> FVRKNPKSDKFKVKRFHHIEFWCGDATNVARRFSWGLGMRFSAKSDLSTGNMVHASYLLTSGDLRFLFTAPYSPSLSAGEIKPTTTASIPSFDHGSCRSFFSSHGLGVRAVAIEVEDAESAFSISVANGAIPSSPPIVLNEAVTIAEVKLYGDVVLRYVSYKAEDTEKS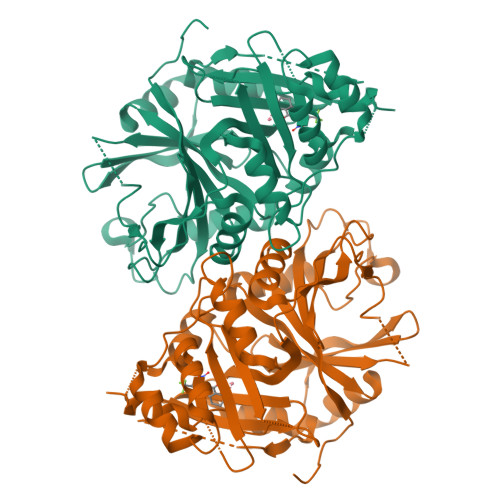EFLPGFERVEDASSFPLDYGIRRLDHAVGNVPELGPALTYVAGFTGFHQFAEFTADDVGTAESGLNSAVLASNDEMVLLPINEPVHGTKRKSQIQTYLEHNEGAGLQHLALMSEDIFRTLREMRKRSSIGGFDFMPSPPPTYYQNLKKRVGDVLSDDQIKECEELGILVDRDDQGTLLQIFTKPLGDRPTIFIEIIQRVGCMMKDEEGKAYQSGGCGGFGKGNFSELFKSIEEYEKTLEAKQLVG>RFYVKDHRNKAMINLHIQKDNPKIVHAFDGEDLGDKAVYCRCWRSKKFPFCDGAHTKHNEETG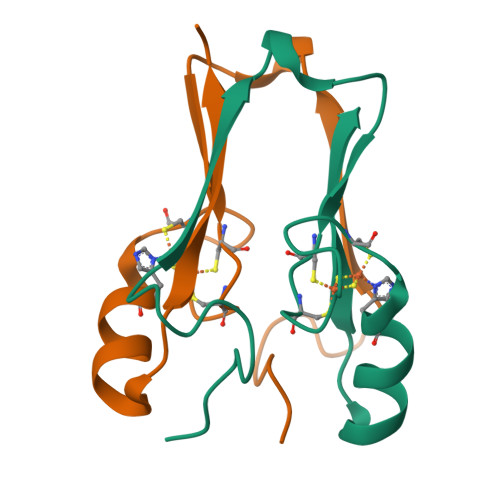DNVGPLIIKKKET[2x]>GSMPLLLDDGDPKAQTGFDLSTATTLFWRPVPVHVKQQDREDVLEELTFRILTGVAKQNHNLRILRIHISSDSDLFFLHTLEVSEEDFQSLKNDQCILVDFASFPGKIISLLEKCILAQPGDSPRFQAVLTIRGGESVFKIVEINDFCQLPHITLAFR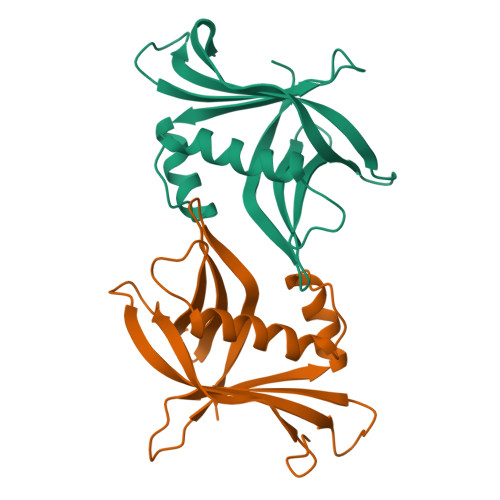PGN[6x]>CGFGGSGSNGEGKKDSKGKTTLNINIKTEPFSLHPGLANDSVSGGVIRQTFEGLTRINADGEPEEGMASKIETSKDGKTYTFTIRDGVKWSNGDPVTAQDFEYAWKWALDPNNESQYAYQLYYIKGAEAANTGKGSLDDVAVKAVNDKTLKVELNNPTPYFTELTAFYTYMPINKKIAEKNKKWNTNAGDDYVSNGPFKMTAWKHSGSITLEKNDQYWDKDKVKLKKIDMVMINNNNTELKKFQAGELDWAGMPLGQLPT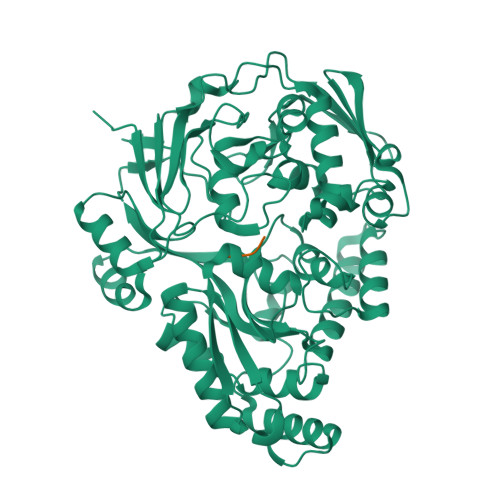ESLPTLKKDGSLHVEPIAGVYWYKFNTEAKPLDNVNIRKALTYSLDRQSIVKNVTQGEQIPAMAAVPPTMKGFEDNKEGYFKDNDVKTAKEYLEKGLKEMGLSKASDLPKIKLSYNTDDAHAKIAQAVQEMWKKNLGVDVELDNSEWNVYIDKLHSQDYQIGRMGWLGDFNDPINFLELFRDKNGGNNDTGWENPEFKKLLNQSQTETDKTKRAELLKKAEGIFIDEMPVAPIYFYTDTWVQDENLKGVIMPGTGEVYFRNAYFK[2x];>[2x]SNSS>MPDNPSTKGRMMRNQQAEHTPVTVIGLGLMGQALAGAFLGAGHPTTVWNRTAAKAEPLVARGAKSAGSVAEAVAASPLVVVCVSDYDAVHALLDPLDGTALQGRTLVNLTSGTSAQARERAAWADGRGADYLDGAILAGPAAIGTADAVVLLSGPRSAFDPHASALGGLGAGTTYLGADHGLASLYDAAGLVMMWSILNGFLQGAA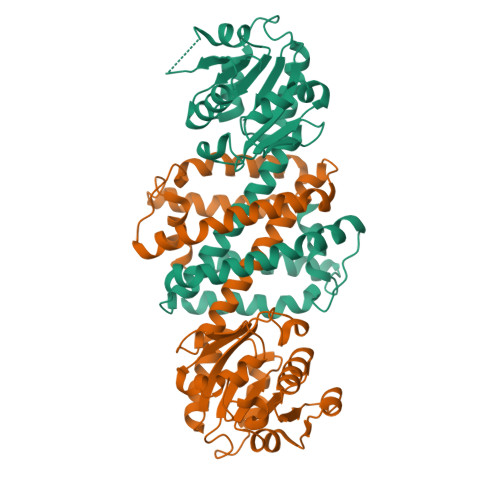LLGTAGVDATTFAPFITQGIGTVADWLPGYARQIDDGAYPADDAAIDTHLATMEHLIHESEFLGVNAELPRFIKALADRAVADGHGGSGYPALIEQFRTHSGK[4x]>[4x]GHMSQPFLWRRVNDSSGFAEPRVFIRVYLEPGSIDAAIAFYEDLQGVAHDMRFDFPEKRLTLAAVGAFLLLEGSDEALAPFRSTTGTLLVDDIEPYHRRLLA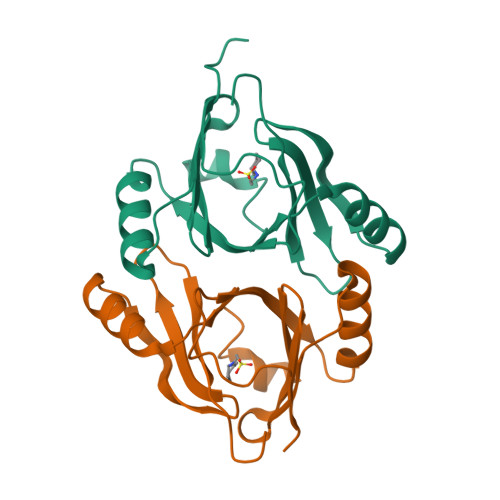AGAQIIFGPARAPTGACFNALLPDGTVVEFVHHRPQPGEA>[2x]APEVSEEPRCPRAACQAKRGDQRCDRECNSPGCGWDGGDCSLSVGDPWRQCEALQCWRLFNNSRCDPACSSPACLYDNFDCHAGGRERTCNPVYEKYCADHFADGRCDQGCNTEECGWDGLDCASEVPALLARGVLVLTVLLPPEELLRSSADFLQRLSAILRTSLRFRLDAHGQAMVFPYHRPSPGSEPRARRELAPEVIGSVVMLEIDNRLCLQSPENDHCFPDAQSAADYLGA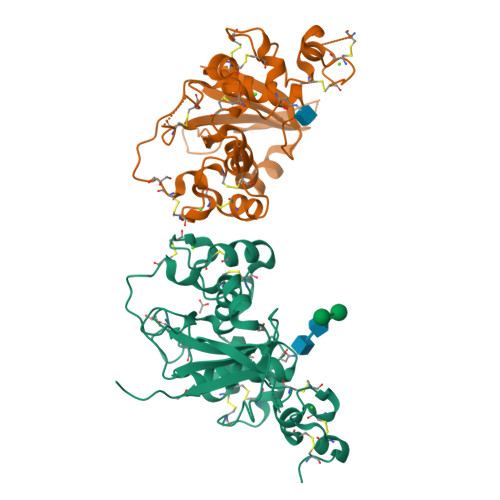LSAVERLDFPYPLRDVRGEPLEPPEPSGSHHHHHH>[2x]IHEGPYPEPL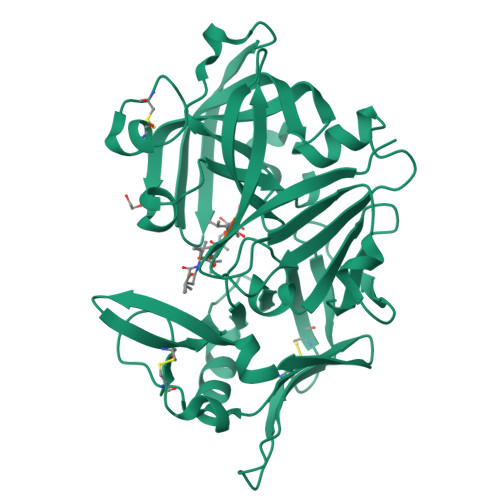VNLLDVVYYGPISIGTPPQDFQVIFDTGSANLWLPSSKCTTKYCLHHHRYDSSKSSTYEADGRNFTIVYGSGNVEGFISKDVCRIGSAKVSGQPLGEALVVGGESLLEAPFDGILGLAYPSIAVDGVVPVFDNMMKQGLLGEQNVFSVYLNRDPSSKEGGEVLFGGIDHDHYKGSITYVPVTAKGYWQFHVDGVKSVSASKSAPELLCKDGCEAIADTGTSLITGPPEEVDSLNQYLGGTKTEGGQYLLDCDKLESLPNVTFTISGKEFSLRSKDYVLKVNQQGQTLCVSGFMGLEMPQPLWILGDVFLGPYYTIFDRDQDRVGFAEVA> KHKILHRLLQDSSSP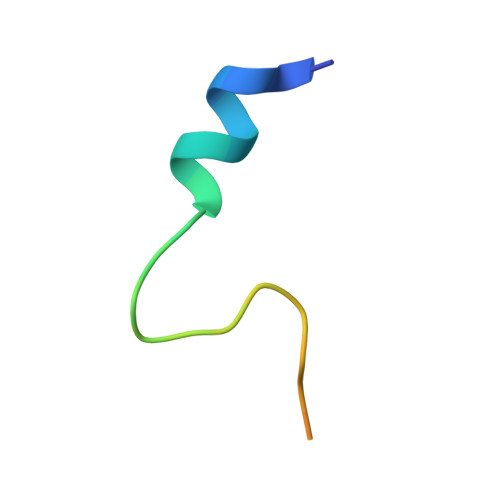VDLAKLTAEATGK> MSDHTRSQNWT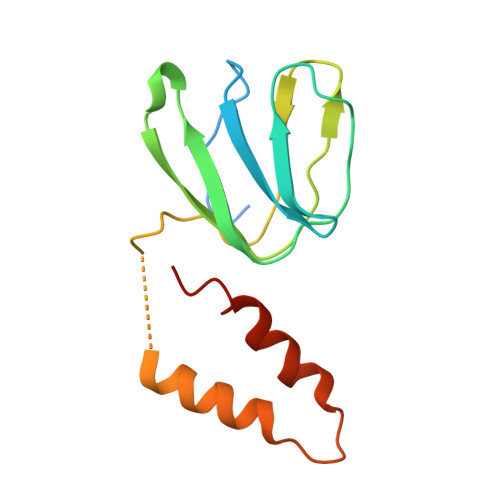NLILTQSIYNQKEVTQVNIPSTAGELGILANHVPTIQQLKPGVVEVIETNGETKSYFISGGFATVQPDSELSVNSIEAFQAEDFSPEAIKSLTAEAQKNAQSADEAVAAEAEIELEVLEALAHFAK>GPLGSMNLIPTVIETTNRGERAYDIYSRLLKDRIIMLGSQIDDNVANSIVSQL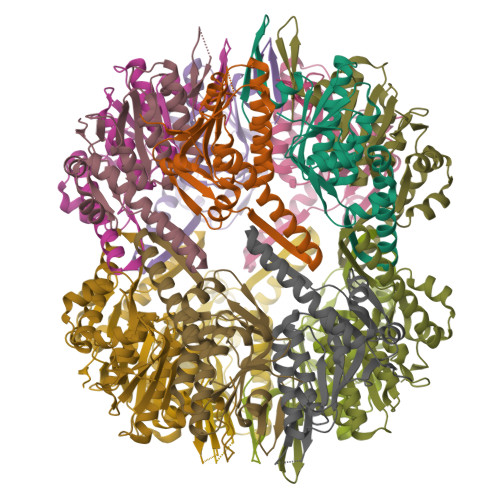LFLQAQDSEKDIYLYINSPGGSVTAGFAIYDTIQHIKPDVQTICIGMAASMGSFLLAAGAKGKRFALPNAEVMIHQPLGGAQGQATEIAIAANHILKTREKLNRILSERTGQSIEKIQKDTDRDNFLTAEEAKEYGLIDEVMVPETK[14x]> TESIPEEMKQIVEEQGNKLHWAALLILMVIIPTIGGNTLVILAVSLEKKLQYATNYFLMSLAVADLLVGLFVMPIALLTIMFEAMWPLPLVLCPAWLFLDVLFSTASIWHLCAISVDRYIAIKKPIQANQYNSRATAFIKITVVWLISIGIAIPVPIKGIETDVDNPNNITCVLTKERFGDFMLFGSLAAFFTPLAIMIVTYFLTIHALQKVRLLSGSRQTISNEQRASKVLGIVFFLFLLMWCPFFITNITLVLCDSCNQTTLQMLLEIFVWIGYVSS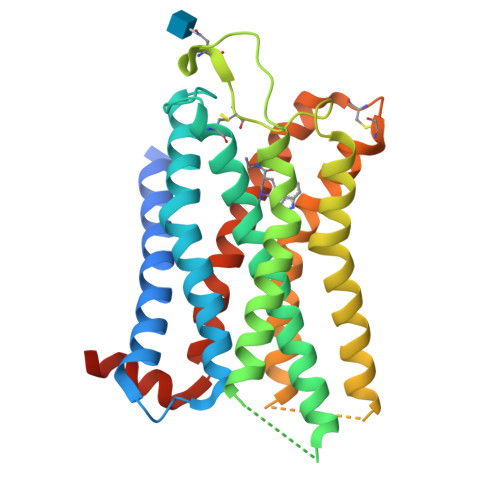GVNPLVYTLFNKTFRDAFGRYITCNYRATKSV> RPSFCNLP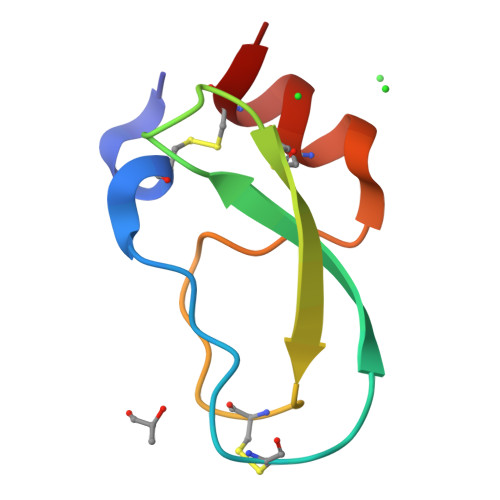VKPGPCKAFFSAFYYSQKTNKCHSFTYGGCKGNANRFSTLEKCRRTCVG> MNGQHPRSVVTAPDATTGTTSYDVVVVGAGIAGLYAIHRFRSQGLTVRAFEAASGVGGVWYWNRYPGARCDVESIDYSYSFSPELEQEWNWSEKYATQPEILAYLEHVADRFDLRRDIRFDTRVTSAVLDEEGLRWTVRTDRGDEVSARFLVVAAGPLSNANTPAFDGLDRFTGDIVHTARWPHDGVDFTGKRVGVIGTGSSGIQSIPIIAEQAEQLFVFQRSANYSIPAGNVPLDDATRAEQKANYAERRRLSRESGGGSPHRPHPKSALEVSEEERRAVYEERWKLGGVLFSKAFPDQLTDPAANDTARAFWEEKIRAVVDDPAVAELLTPKDHAIGAKRIVTDSGYYETYNRDNVELVDLRSTPIVGMDETGIVTTGAHYDLDMIVLATGFDAMTGSLDKLEIVGRGGRTLKETWAAGPRTYLGLGIDGFPNFFNLTGPGSPSVLANMVLHSELHVDWVADAIAYLDARGAAGIEGTPEAVADWVEECRNRAEASLLNSANSWYLGANIPGRPRVFMPFLGGFGVYREIITEVAESGYKGF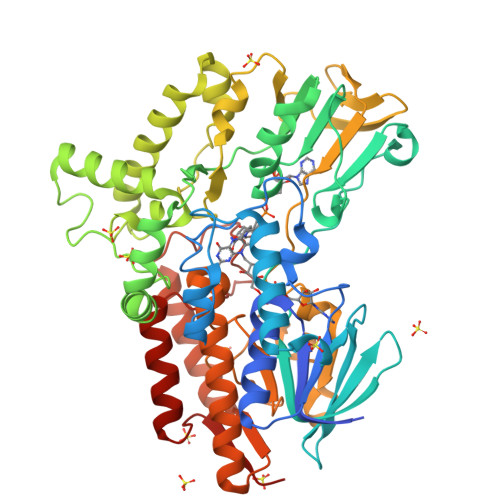AILEG>MSVIKSDMKIKLRMEGTVNGHKFVIEGEGEGKPYEGTQTMNLKVKEGAPLPFAYDILTTVFHYGNRVFTKYPKHIPDYFKQSFPEGYSWERSMTFEDGGICTARNDITLEGDCFFNEIRFDGVNFPPNGPVMQKKTLKWEPSTEKMYVRDGVLTGDINMALLLEGGGHYRCDFKTTYKAKKGVQLPDYHFVDHCIEILSHDKDYNNVKLYEHAVAHSGLPRQAKHHHHHH[4x]

LEA was engineered to represent the evolutionary node that acquired the unique ability to photoconvert from the ancestral green fluorescent protein (ALL-GFP), which was engineered on the basis of ancestral gene reconstruction from the great star coral Montastraea cavernosa. Perhaps the most important mutation to make LEA photoconvertible is modifying the chromophore to a His-Tyr-Gly (HYG) chromophore, making it a Kaede-type FP. Another green-to-red pcFP named the least-evolved ancestor (LEA) was also discovered to display pronounced photoswitching of both the green and red forms. Several photoconversion mechanisms have been proposed for the Kaede-like pcFPs, and most mechanisms involve a β-elimination reaction and backbone breakage to extend the conjugation between Gly64 and His62 that forms the red chromophore, although the complete photocycle remains largely unanswered.

A notable reverse single-site mutant (LEA-A69T) involves modifying Ala69 back to Thr69, which ALL-GFP and ALL-Q62H both possess. The A69T mutation has been documented to cause large pK a changes, which is clearly the case for LEA-A69T (pK a = 8.4) versus LEA (pK a = 6.3). Interestingly, LEA-A69T is not photoswitchable under 505 nm illumination (blue), which is considered to be a marker for a primed-convertible FP. LEA-A69T crystallized in space group P212121 with a full tetramer in the asymmetric unit, while LEA-H62X crystallized in I222 with a single protomer per asymmetric unit; both crystal forms were described previously for LEA. In contrast, with a slightly twisted P-ring conformation, LEA-A69T displays the lowest FQY of 0.73 upon 490 nm excitation. The lack of photoswitching in LEA-A69T is likely influenced by the π-stacked His193 that helps to maintain bright fluorescence of the anionic green chromophore. In LEA-A69T, His193 is slightly shifted horizontally resulting in a larger angle between the two rings yet maintaining a closer ring-to-ring distance of 3.7 Å. In particular, Thr69 causes Arg66 to reorient and H-bond to the bulkier Thr69 in LEA-A69T and ALL-Q62H, instead of the I-ring C=O group in LEA and LEA-H62X via the reoriented Arg66 without an H-bond to the smaller Ala69. In contrast, the distances within the internal charge network change drastically in LEA-A69T due to the Thr69-induced changes, wherein the distances between Glu144 and Arg66 increases from 4.4 to 6.2 Å (due to the reoriented Arg66) and the distance between Glu211 and His193 increases from 2.6–2.7 Å to 3.3 Å, while the Arg66 to Glu211 distance shrinks from 4.4–4.6 Å to 2.8 Å. Such a shortened distance between Arg66 and the catalytic base Glu211 (highly conserved among LEA FPs) and the resultant disruption to the internal charge network may underlie the significantly hindered photoconversion of LEA-A69T; however, more rationales need to be developed for the further reduction of photoconversion efficiency in LEA-H62X.> MTDALGIDKELNLKKKQRAPKVKLDDQRLLSEKGIPKLRKMAPRLKFKGKGHEFSDTARLLSFYQEWLDDLFPKATFLDALAMVEKAGHKTTVRNARLKWIDEL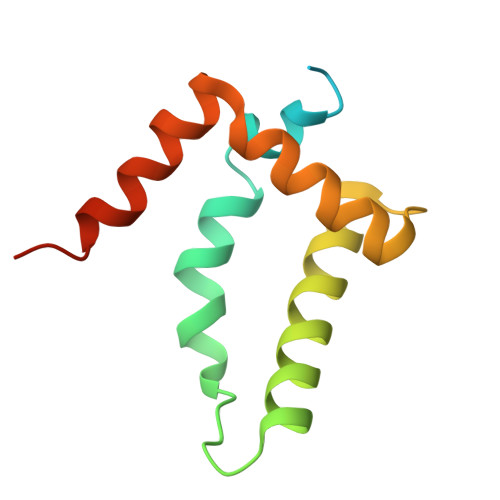RPKASFE>QSKQGATYDFTPLDSIISSWMDKGYYPGGAICVVKNDSVLFEKAYGSFTGDTKVYVASAGKWVAAAVIGAVVDRTDLSWDDPVEKWLPQFRGDAKGGILLRQLLSHTSGVRPYLPAPRVDNYNHLDSAVTEILSLDTVFTPGTRFEYGGLAMQIAGRMAEVAMGKEFEPLFQELIAAPLGMTHSHFAPVNTDGGHAPMLGGGLCTTLNDYIRFLKMIYHNGRSGNREILKPETVQTMQADQVRNAVVAPGEYVEKALGQHHTSIYGLGEWRELVDEATGEAYQISSPGWAGAYPWINKRDGVYGFFIAHVQGEAN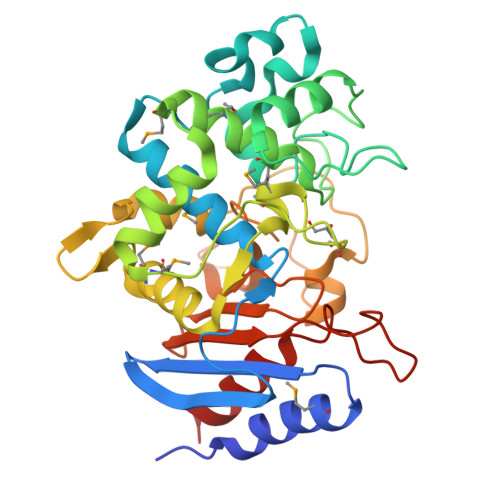KKDGFSSFYGSPVLSETVTKIVNQ[4x]> MMRRVASTGSNGGHCYVGSSLWADSVYMEVSSITLQKRFSFKYATKLQHDEMRQPYYIHEKRYGIFSNERNIAKARRGLPFITPLYTKHMNLWDTDTDASNNRFFRGYYYGQRELHQLLGRPHSLEATNADGSNDLSTYEANTSQLYKGIPRPAITNLHYEPAWRYTLYQAGAHGAQLSNPRSPFTAKVLGDELMQVRDIKSVEHCKAWFDRLQYLINLHYEAVGDIGEFKSRHTRHVHEFFVAFHDALSSLDFRDTYLFDQFKAVRPPELSDLFGIFLEMEANYVHEDYCPRCSLPYSTTRYCGEGDVDTPFRKHRGRWAPHQKWGREWYDVVARRAEALWYRATEDPYFGTPQHTQRQAEALLKVYVQAKQRGKAIDFMNKLRGSVEYLTGDITITTVMQESYDALLDTTPHPHLLTNGFTLESDAAKYTGEVNKAPLSPLQFRIDMEMNKYRRQQKEEGVVRVPPALWRLDTSAIVPYKVDSKTRRIVNWREVKEGIEKSFLSVGLPKEAYTGNEWREMLYLHDVIANREAKAAVLEQQQKLDREKLKARERASLKGEKSSNSASNGIGIIFPDKDGYQVFFVDEASLRPFGIGASGTLFKAVARVYPSPAAVPYDDPVHGKQFLIDTTDETCHLFGGFEHGDRLLLRAKSSGGDVDGGNNSNCRNTGSFTDEEEEVIVMGVSTEGSDAERMLCAMHVDTGKQRERGIVFLGTDCIDIRERWESVRYAASAYVKGRVTLLESQRTAREEFMGQVVGIRDGVLFVQWRLLKGGGSVLDRSVAVPIGDSTQVRELFVETKVLGVEPLQSPPSWRTPFRNDFAEERLKELQRAPFKREKYVSLIQGKYTPKVKKFGYTQHTTVDDFETKEYKDRLLSKQFFQNPQAFEVVPDRHERSVQFGGKWEYQRTHGLPTVDRNELENGWSEVEPISDGEMKVIEQALRDISGPRPGNFVKPPSKTKSLQLSESWWEPLGYGWEQHNEEQKALCDVTEQRLIDGSNLPFGGKLPPFGTSYGMGERMRAIIEDYSKGFGLGPHGHSPTHDTIHYNTLNAEGERVRDLGYTDALGRLFSEKLGDRDVHQWAVESCADGEADVRQLLLSLHEWRERGRPPSLLLANVLSKYLEEEIAAFNKGIPENAPKLQLETSDGTLAHSGSGGSRSGTMWADVDPTTFALHQASQSTRSTRCDEPFILHLVKRAKLGECVTNFTDTAYIAHLESSVINEFHLALTKLVGKGISPTLLAQKTGQLHRGSVRVGGNVVPFVKSRELSRLLERMGLTSESIAVITRGLANCPEQESVGDDFAVPVSLILSWDGPGSSGGSGSGDRRLNTTAARNEQQRKGSAALSSAIRQLSQHQKQRGSASGRGWQNEDKMVVHVLEELSLRNDGLVMDIQYAIRENKKNRRLRWEFVTTLLPVFGGNEAKVEQLYSDYCDGKYVPNITVAVEAFIAFLHNATQHPETYSASDYFDIDDGKSSTASGTGDQPSAGQYTTLKLLDPLEGPFVFDNVKVEYIQTVERFRRHGIRAGPVMAPATGFIAANCKSLNYFTRRQEEVVYVTNDSDQGLRRSLENSAYHKTIAANPALQYLLKARRGAALV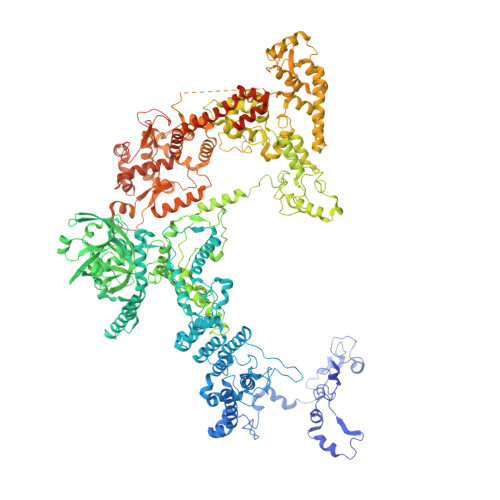ETFNRFFYRTMPMLNFYQNVLKHYSETIQPLRQAAKSSTRGLARALESERSAAMEEFRRNSERYWRNIIEGRSVEQVVLANGESNRRTVGGGAGEQLQKPQGNRDAVRTNFTGEATDGSRKGQRQHQQPPLSQQQQHSRGEGERSAVHTSPRQGGSRGMADLLSKLNTPKTGSGVKGSTAKNTGNNRRGPKS> MAFEENLYCDYTPGA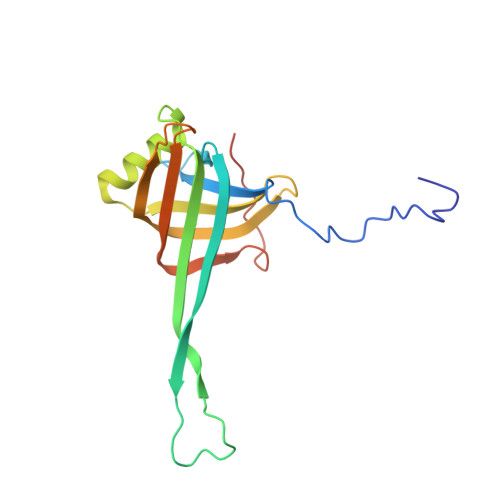AKAVAGKDVILAVFNAAGDKLLAVAGQQGLTVNRSKDSIEITSKDTVGGWKSKIGGMKEWSIENDGLYVADAESHKELAKYFESDSPVCVKIINQASKKGLFGGLAIVADYSFEAPFDEAMTYSVKLDGMGALVDLTITEGGDQMPGETPVAPAE Excessive replication of Saccharomyces cerevisiae Ty1 retrotransposons is regulated by Copy Number Control, a process requiring the p22/p18 protein produced from a sub-genomic transcript initiated within Ty1 GAG. To minimize genomic damage, p22/p18 interrupts virus-like particle function by interaction with Gag. Thus, p22 is identical to the C-terminal half of Gag-p49 and is processed at the C-terminus by PR to generate a mature protein p18, that is identical to the C-terminal half of mature capsid Gag-p4525,27. The structure comprises an all α-helical domain related to that observed in the CA-CTD of the yeast Ty3 retrotransposon, ARC proteins, and orthoretroviruses.

To further examine the effects of the A273V mutation, we determined the crystal structure of p18mAUG2-A273V. The protein crystallised in the same spacegroup as p18m with the same three copies arranged as two dimers in the ASU, but now with additional electron density for the A to V substitution on α1. Superposition of the three monomers shows the backbone conformation is near identical (RMSD = 0.16 ± 0.04 Å over 78 ± 3.6 Cα) as was also observed with WT p18m. In addition, the Dimer-1 interface contains the same set of apolar and H-bond interactions as in the WT structure. The only difference is the alanine to valine substitution located at the interface centre. In p18m-A273V, it is apparent that the γ-methyl groups of V273 now also form part of the continuous apolar network. However, in order to accommodate the additional methyl groups, there is a small displacement in the backbone position at the C-terminus of α1 in both monomers. As a result of this shift, the V273 γ-methyl groups also pack across the dimer interface and maintain the same favourable 3.6 Å Van der Waals spacing as the β-methyl groups of A273 in the p18m structure. Analysis of the energetic contribution from A273 or V273 to the dimer interface using PDBePISA52 also suggests that both the A273–A273 and V273–V273 interactions are favourable and that V273–V273 packing actually contributes more than the A273–A273 packing to the free energy of the overall interaction. However, analysis of Tm derived from derivative plots gives values of 50.7 ± 0.4 °C for p18m and 45.8 ± 0.2 °C and 45.1 ± 0.3 °C for A273V and I269F mutants respectively, showing that these amino acid substitutions modestly reduce protein stability.

>MQSDTQEANDIVTLVNLQYNGSTPADAFETKVTNIIDRLNNNGIHINNKVACQLIMRGLSGEYKFLRYTRHRHLNMTVAELFLDIHAIYEEQQGSRNPLEHHHHHH[3x]>SMGNMCMVMFGYDMIHITVFQPDKSRSEYCDEIPATGRTIMAFDIENPAFRDLPLELRIIRDPLTPVLPTGEKELDALTELHLPAKKYSKGTFSVEHNFANNGHYIGLVTLTRESGQQETAQFKFMVG[2x]

PmoD/AmoD represent a family of copper-binding proteins specific to MOB and AOB, the key players in global carbon and nitrogen cycling. Sequence analysis indicates that PmoD/AmoD comprises an N-terminal signal peptide followed by a periplasmic domain containing two strictly conserved cysteine residues and a C-terminal transmembrane helix within the inner membrane. Here we show that PmoD forms a copper center exhibiting the features of a CuA site using a previously unobserved ligand set at the interface of a PmoD homodimer. We further show that PmoD is critical for the copper-dependent growth of Methylosinus trichosporium OB3b on methane.

We heterologously expressed and purified the periplasmic domain of PmoD encoded by the Methylocystis species (sp.) strain Rockwell extended pmo operon (PmoDMet49242_1452; there are 10 other pmoD genes in the genome of this species). The copper ion is coordinated in tetrahedral geometry by Met42 and Met44 from each monomer, and the two invariant cysteine residues, Cys41 and Cys65, form an intramolecular disulfide bond. Given that the crystals were obtained from the monomeric PmoDMet49242_1452 species, it is likely that the observed copper-binding site is a crystallization artifact. The PmoDMet49242_1452 structure differs from these canonical CuA domain structures in three distinct regions. First, the N-terminal histidine ligand in the Hx34Cx3Cx3Hx2M CuA motif typically derives from the loop between β3 and β4, but PmoDMet49242_1452 contains a small helix in place of this loop and lacks a histidine in the equivalent position. Second, the loop between β7 and β8 provides the other four CuA ligands, but PmoDMet49242_1452 lacks not only this sequence motif, but also any histidine, cysteine, or methionine residues in this area. Finally, the N-terminal region of PmoDMet49242_1452 diverges in the orientation of β1 and β2, as well as the presence of an additional β strand prior to β1. Instead of the canonical CuA ligands, PmoDMet49242_1452 contains a cluster of surface-exposed cysteine, methionine, and histidine residues near its N terminus, including the universally conserved cysteine residues Cys41 and Cys65. Thus, despite the overall similarity in fold to other CuA domains, the PmoD CuA site is formed by two protein molecules and a completely different part of the protein structure in contrast to all previously characterized CuA centers which are housed within a single cupredoxin domain.>[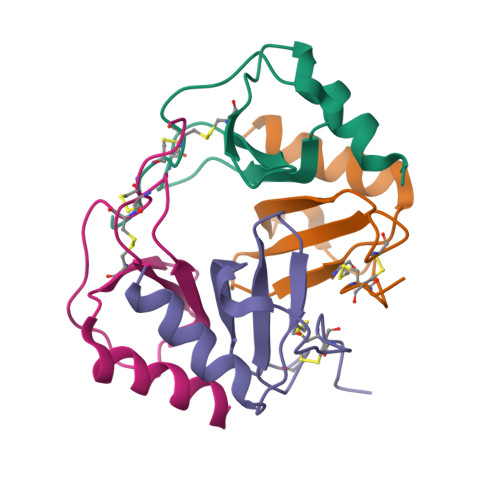4x]EAEEDGDLQCLCVKTTSQVRPRHITSLEVIKAGPHCAVPQLIATLKNGRKICLDLQAPLYKKIIKKLLES>MAFYKREMFDPAEKYKMDHRRRGIALIFNHERFFWHLTLPERRGTCADRDNLTRRFSDLGFEVKCFNDLKAEELLLKIHEVSTVSHADADCFVCVFLSHGEGNHIYAYDAKIEIQTLTGLFKGDKCHSLVGKPKIFIIQ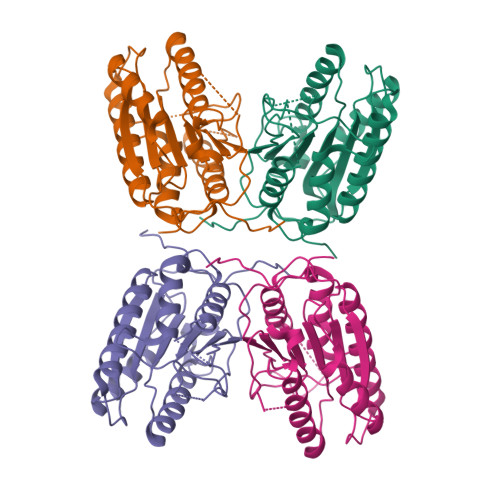ACRGNQHDVPVIPLDVVDNQTEKLDTNITEVDAASVYTLPAGADFLMCYSVAEGYYSHRETVNGSWYIQDLCEMLGKYGSSLEFTELLTLVNRKVSQRRVDFCKDPSAIGKKQVPCFASMLTKKLHFFPKSNHHHHHH[4x]methyl 3-[(thiophen-2-ylacetyl)amino]thiophene-2-carboxylate | 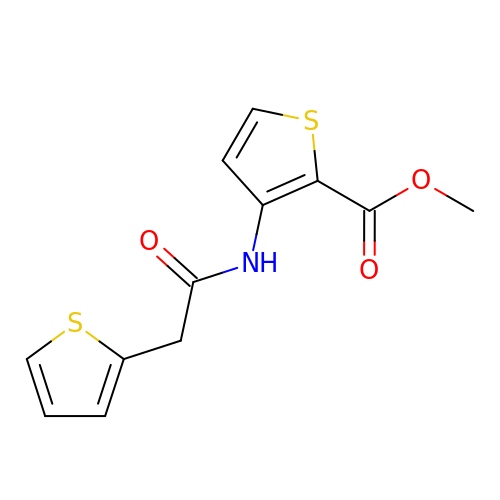C12 H11 N O3 S2 | CXOCENPNQSXLGZ-UHFFFAOYSA-N> GSMDTSGKQAEAMALLAEAERKVKNSQ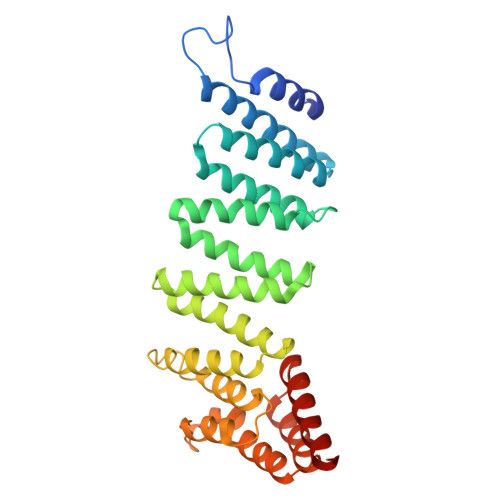SFFSGLFGGSSKIEEACEIYARAANMFKMAKNWSAAGNAFCQAAQLHLQLQSKHDAATCFVDAGNAFKKADPQEAINCLMRAIEIYTDMGRFTIAAKHHISIAEIYETELVDVEKAIAHYEQSADYYKGEESNSSANKCLLKVAGYAAQLEQYQKAIDIYEQVGTSAMDSPLLKYSAKDYFFKAALCHFCIDMLNAKLAVQKYEELFPAFSDSRECKLMKKLLEAHEEQNVDSYTESVKEYDSISRLDQWLTTMLLRIKKTIQGDEEDLR>MTEEKKLWQKGGGWLLEVPERVYTPEDFDESVKEIARTTRTFVEREVLPLLERMEHGELELNVPLMRKAGELGLLAIDVPEEYGGLDLPKVISTVVAEELSGSGGFSVTYGAHTSIGTLPLVYFGTEEQKRKYLPKLASGEWIAAYCLTEPGSGSDALAAKTRATLSEDGKHYILNGVKQWISNAGFAHLFTVFAKVDGEHFTAFLVERDTPGLSFGPEEKKMGIKASSTRQVILEDVKVPVENVLGEIGKGHKIAFNVLNVGRYKLGAGAVGGAKRALELSAQYATQRVQFGRPIGRFGLIQQKLGEMASRIYAAESAVYRTVGLIDEALLGKKGPEAVMAGIEEYAVEASIIKVLGSEVLDYVVDEGVQIHGGYGYSQEYPIERAYRDARINRIFEGTNEINRLLIPGMLLRRALKGQLPLMQAAQRLQKELLEPSFEEPEDLELHQVQNLKKLALMVAGLAVQKYGQGVEEEQEVLGAVADILIDAYAAESALLRARRLGGLAPVLARIYLAQALDRAQAGALSVLPRLVEGDEARVVYSAARRLTKREPGDLVALRRQAAEAVLEAGG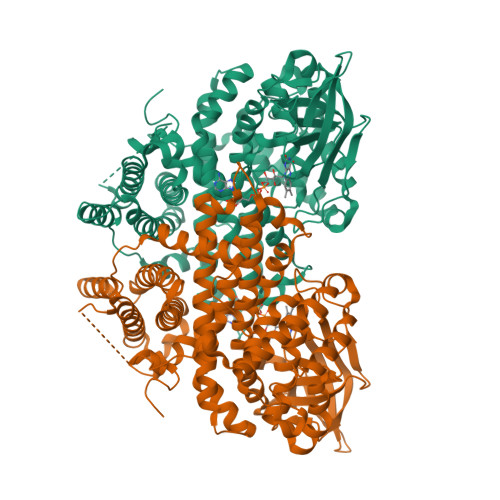YPIPR[2x]> LQR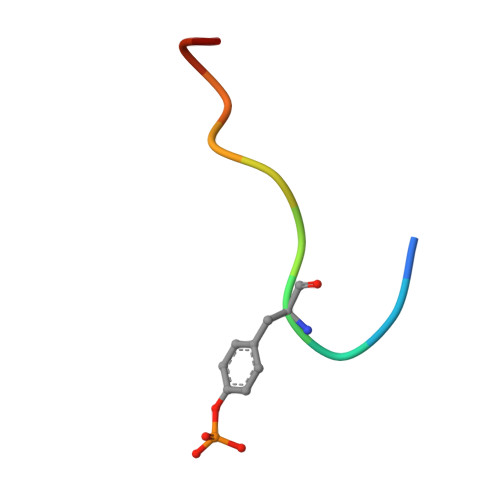YSSDPTGA>[6x]SKSDVFHLGLTKNDLQGAQLAIVPGDPERVE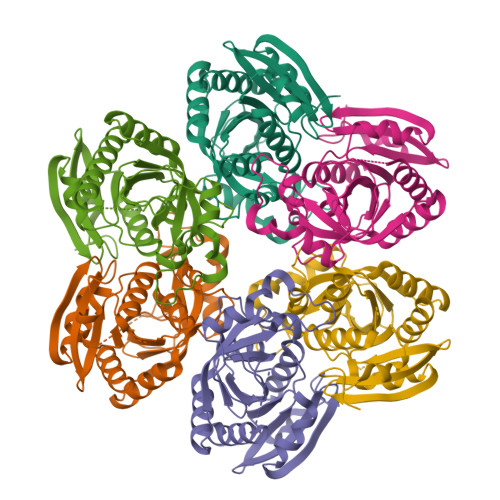KIAALMDKPVKLASHREFTSWRAELDGKAVIVCSTGIGGPSTSIAVEELAQLGIRTFLRIGTTGAIQPHINVGDVLVTTASVRLDGASLHFAPMEFPAVADFACTTALVEAAKSIGATTHVGVTASSDTFYPGQERYDTYSGRVVRRFKGSMEEWQAMGVMNYEMESATLLTMCASQGLRAGMVAGVIVNRTQQEIPNAETMKQTESHAVKIVVEAARRLL> QNRTVKGTVISSEDNEPLIGANVVVVGNTTIGAATDLDGNFTLSVPANAKMLRVSYSGMTTKEVAIANVMKIVLDPDSKVLEQVVVLGYGTGQKLSTVSGSVAKVSSEKLAEKPVANIMDALQGQVAGMQVMTTSGDPTAVASVEIHGTGSLGASSAPLYIVDGMQTSLDVVATMNPNDFESMSVLKDASATSIYGARAANGVVFIQTKKGKMSERGRITFNASYGISQILNTKPLDNMMTGDELLDFQVKAGFWGNNQTVQKVKDMILAGAEDLYGNYDSLKDEYGKTLFPVDFNHDADWLKALFKTAPTSQGDISFSGGSQGTSYYASIGYFDQEGMAREPANFKRYSGRLNFESRINEWLKVGANLSGAIANRRSADYFGKYYMGSGTF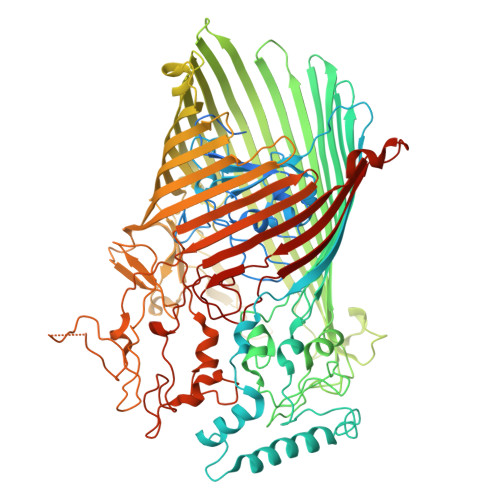GVLTMPRYYNPFDVNGDLADVYYMYGATRPSMTEPYFAKMRPFSSESHQANVNGFAQITPIKGLTLKAQAGVDITNTRTSSKRMPNNPYDSTPLGERRERAYRDVSKSFTNTAEYKFSIDEKHDLTALMGHEYIEYEGDVIGASSKGFESDKLMLLSQGKTGNSLSLPEHRVAEYAYLSFFSRFNYGFDKWMYIDFSVRNDQSSRFGSNNRSAWFYSVGGMFDIYNKFIQESNWLSDLRLKMSYGTTGNSEIGNYNHQALVTVNNYTEDAMGLSISTAGNPDLSWEKQSQFNFGLAAGAFNNRLSAEVDFYVRTTNDMLIDVPMPYISGFFSQYQNVGSMKNTGVDLSLKGTIYQNKDWNVYASANFNYNRQEITKLFFGLNKYMLPNTGTIWEIGYPNSFYMAEYAGIDKKTGKQLWYVPGQVDADGNKVTTSQYSADLETRIDKSVTPPITGGFSLGASWKGLSLDADFAYIVGKWMINNDRYFTENGGGLMQLNKDKMLLNAWTEDNKETDVPKLGQSPQFDTHLLENASFLRLKNLKLTYVLPNSLFAGQNVIGGARVYLMARNLLTVTKYKGFDPEAGGNVGKNQYPNSKQYVAGIQLSF>[2x]ATPWQKITQPVPGSAQSIGSFSNGCIVGADTLPIQSEHYQVMRTDQRR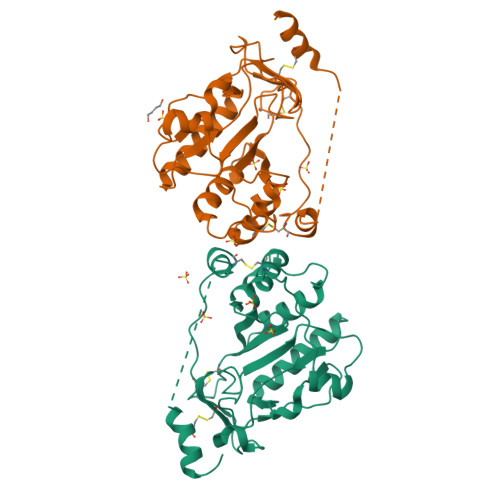YFGHPDLVMFIQRLSSQVSNLGMGTVLIGDMGMPAGGRFNGGHASHQTGLDVDIFLQLPKTRWTSAQLLRPQALDLVSRDGKHVVSTLWKPEIFSLIKLAAQDKDVTRIFVNPAIKQQLCLDAGTDRDWLRKVRPWFQHRAHMHVRLRCPADSLECEDQPLPPSGDGCGAELQSWFEPPKPGTTKPEKKTPPPLPPSCQALLDEHVI The Japanese encephalitis virus is a flavivirus transmitted by Culex mosquitoes and is closely related to other serious emerging viruses, including the dengue virus (DENV), the West Nile virus (WNV), and the Zika virus (ZIKV). The nucleocapsid is composed of multiple copies of the capsid protein, enclosing the single-stranded RNA genome. C proteins have roles, including, but not limited to, nucleocapsid dissociation and assembly. The JEV capsid protein has a helix-rich structure and forms a stable homodimer similar to other flaviviruses.

Here, we present the JEV capsid protein structure at 1.98 Å resolution. Similarly, electron density for the first 25 residues from the JEV C protein N-terminus is not visible in our crystal structure due to cleavage during protein purification. The purified JEV capsid protein, whose size was reduced to less than 15 kDa, was crystallized, and the solved structure has a visible electron density for residues 26–98. Each monomer of the JEV capsid protein is composed of four helices: α1 (amino acid 29–38), α2 (44–57), α3 (63–70), and the longest α4 (74–96), connected by short loops. As is the case for the DENV, WNV, and ZIKV capsid proteins, the JEV capsid protein is a dimer, created by anti-parallel pairing of the α1-α1’, α2-α2’, and α4-α4’ helices, connected by extensive hydrophobic interactions, hydrogen bonds, and salt bridges. The JEV capsid dimer is connected by 13 hydrogen bonds, similar to the ZIKV capsid, with an average distance of 3.06 Å and 2.87 Å, respectively. Almost half of the amino acids of the JEV capsid, of which 41 are residues from the first subunit and 43 are residues from the second subunit, are involved in creating the hydrophobic dimer interface. The large hydrophobic patch on the monomer surface that mediates dimerization is concealed after protein dimerization and the rest of the surface is hydrophilic. The α1-α1’ helices of the JEV, WNV, and ZIKV are found on top of the α2-α2’ helices and protect the hydrophobic surface of α2-α2’, thereby forming a closed conformation. In this study, we crystallized the JEV capsid at pH 4.6, 5.6, and 6.2, each in similar crystal form with identical protein conformation.

>[2x]AMADIGSMTKKPGGPGKNRAINMLKRGLPRVFPLVGVKRVVMSLLDGRGPVRFVLALITFFKFTALAPTKALLGRWKAVEKSVAMKHLTSFKRELGTLIDAVNKRGRKQNKR>GHFKDPKRLYCKNGGFFLRIHPDGRVDGVREKSDPHIKLQLQAEERGVVSIKGVSANRYLAMKEDGRLLASKSVTDECFFF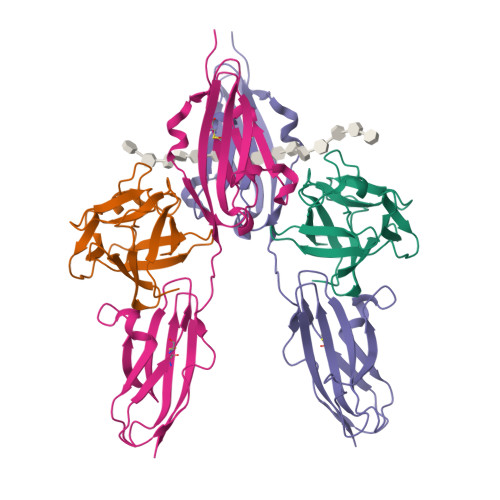ERLESNNYNTYRSRKYTSWYVALKRTGQYKLGSKTGPGQKAILFLPMSAKS[2x];>TDNTKPNRMPVAPYWTSPEKMEKKLHAVPAAKTVKFKCPSSGTPQPTLRWLKNGKEFKPDHRIGGYKVRYATWSIIMDSVVPSDKGNYTCIVENEYGSINHTYQLDVVERSPHRPILQAGLPANKTVALGSNVEFMCKVYSDPQPHIQWLKHIEVNGSKIGPDNLPYVQILKTAGVNTTDKEMEVLHLRNVSFEDAGEYTCLAGNSIGLSHHSAWLTVLEALEER[2x]>MGSSHHHHHHSSGRENLYFQGMTKPLILASQSPRRKELLDLLQLPY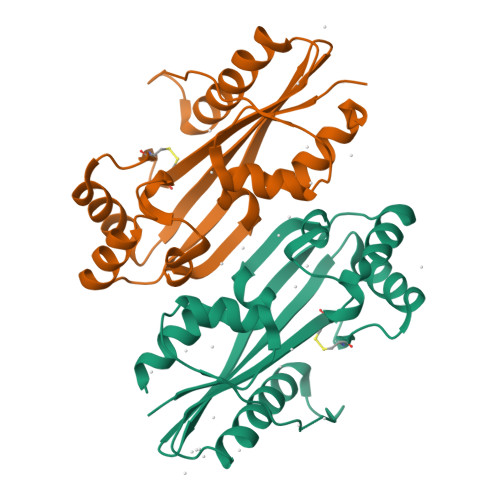SIIVSEVEEKLNRNFSPEENVQWLAKQKAKAVADLHPHAIVIGADTMVCLDGECLGKPQDQEEAASMLRRLSGRSHSVITAVSIQAENHSETFYDKTEVAFWSLSEEEIWTYIETKEPMDKAGAYGIQGRGALFVKKIDGDYYSVMGLPISKTMRALRHFDIRA[2x]> ADPAYFSQFSMRAPDHDPCHDHTGRPVRCVPEFINAAFGKPVIASDTCGTNRPDKYCTVKEGPDGIIREQCDTCDARNHFQSHPASLLTDLNSIGNMTCWVSTPSLSPQNVSLTLSLGKKFELTYVSMHFCSRLPDSMALYKSADFGKTWTPFQFYSSECRRIFGRDPDVSITKSNEQEAVCTASHIMGPGGNRVAFPFLENRPSAQNFENSPVLQDWVTATDIKVVFSRLSPDQAELYGLSNDVNSYGNETDDEVKQRYFYSMGELAVGGRCKCNGHASRCIFDKMGRYTCDCKHNTAGTECEMCKPFHYDRPWGRATANSANSCVACNCNQHAKRCRFDAELFRLSGNRSGGVCLNCRHNTAGRNCHLCKPGFV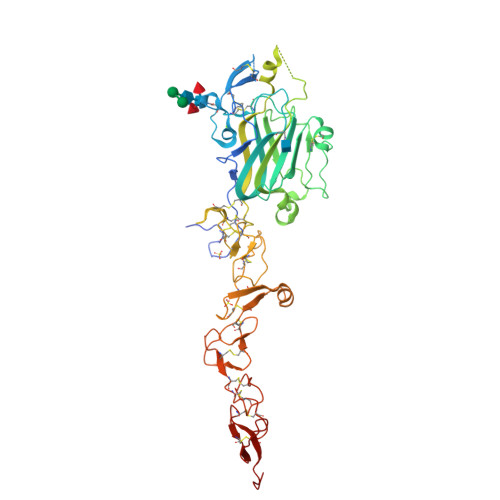RDTSLPMTHRKACKSCGCHPVGSLGKSCNQSSGQCVCKPGVTGTTCNRCAKGYQQSRSTVTPCIKIPHHHHHH quinoxalin-5-ol | C8 H6 N2 O | 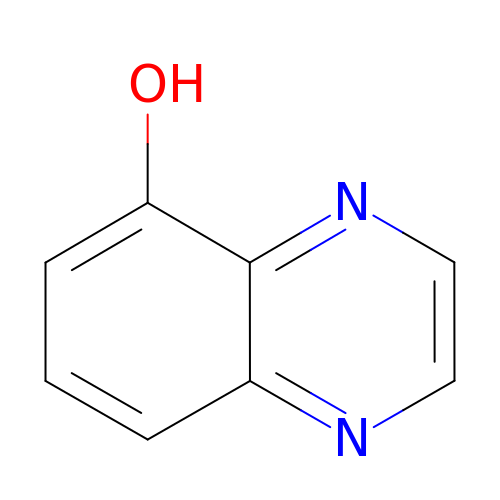ZUQDDQFXSNXEOD-UHFFFAOYSA-N> SLDPTVHWLFTTCGASGPHGPTQAQCNNAYQNSNLSVEVGSEGPLKGIQIWKVPATDTYSISGYGAAGGKGGKNTMMRSHGVSVLGIFNLEKDDMLYILVGQQGEDACPSTNQLIQKVCIGENNVIEEEIRVNRSVHEWAGGGGGGGGATYVFKMKDGVPVPLIIAAGGGGRAYGAKTDTFHPERLENNSSVLGLNGNSGAAGGGGGWNDNTSLLWAGKSLQEGATGGHSCPQAMKKWGWETRGGFGGG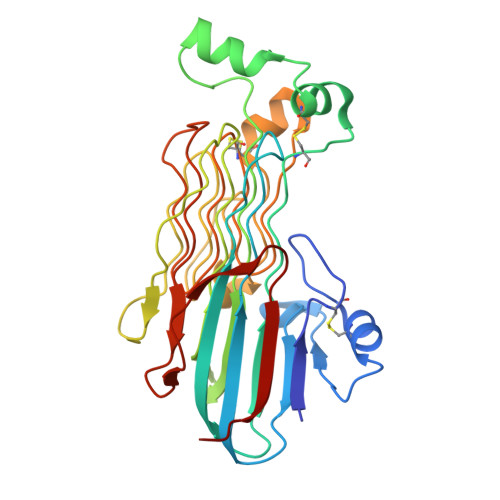GGGCSSGGGGGGYIGGNAASNNDPEMDGEDGVSFISPLGILYTPALKVMEGHGEVNIKHYLN> MGSSHHHHHHSSGENLYFQGHMVDLRSDTVTRPGPAMRRAMAEAVVGDDDYGEDPTVHELQEKAAELLGVERTLF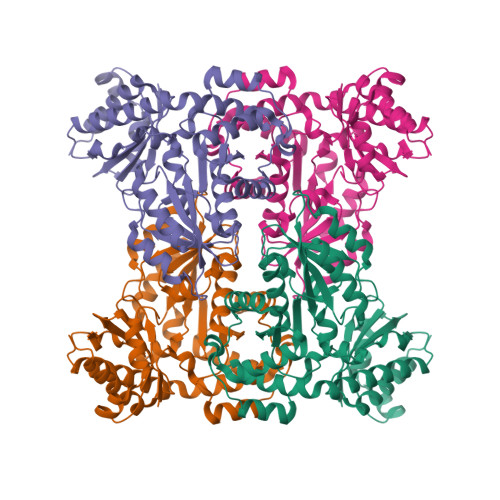VPTNTMANLISVMGHCRRRGSQVLLGQECHLHVYEQGGVAQIAGVHSHPLPDLPYGTLDLNELERALTRGSGSPYHPVCELVYLENTHSSAGGRVLPVDYLRQVCLLAHAHGARVHMDGARLMNAAVALRIPPARLVEHCDSVSFCFSKGLGAPVGALVGGSKDFIGEAWRLRKALGGGMRQAGVLAAAALVGLAEAEEVLPRDHENAQRFAKGLQDLASPICSVDPATVETNMVLVQVAGLPPSELCQRLQAVSAEEVAQTGRAVRVLLFPWTEQSVRAVWHRDVSAQDTELALKKWEFVLRQLRP>[3x]GPMATRGRPRAFDRDTALQRAMDVFWVRGYEGASLAALTEAMEIRPPSLYAAFGSKEGLF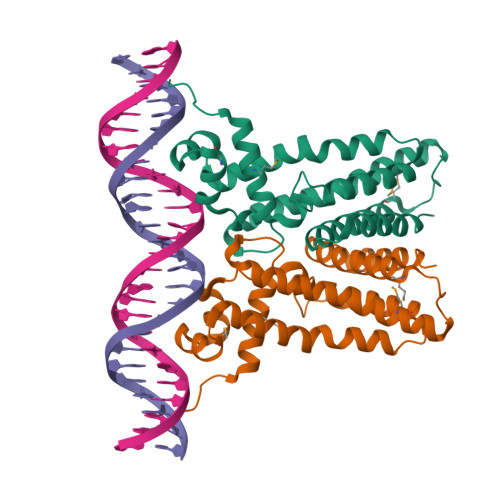REALAHYLGQHGRYRRDVLDGAPSAREGVAELLRETVARFTSDEFPRGCLVVLAALTGTPESEAVRDALSAERGESIRLFRERMRRGIADGDLAADTDMEELATFYATVLFGLSVQAKDRVPRERLLAVVERALRAWP2,4,6,7,8,9-HEXAHYDROXY-5-METHYLCARBOXAMIDO NONANOIC ACID | C11 H21 N O9 | 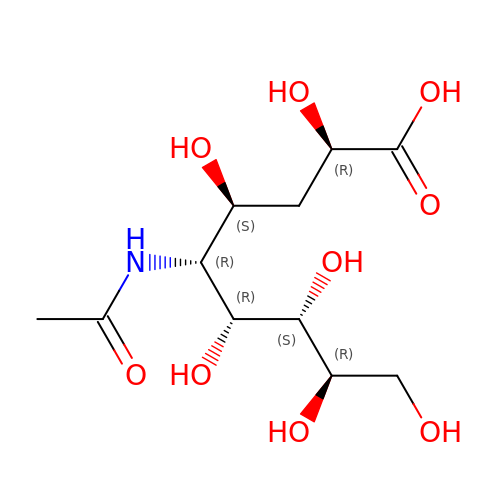REORMAHRVILHOU-IHICSVBISA-N> GSHMLEMIIKPRVRGFICVTAHPTGCEANVKKQIDYVTTEGPIANGPKRVLVIGASTGYGLAARITAAFGCGADTLGVFFERPGEEGKPGTSGWYNSAAFHKFAAQKGLYAKSINGDAFSDEIKQLTIDAIKQDLGQVDQVIYSLASPRRTHPKTGEVFNSALKPIGNAVNLRGLDTDKEVIKESVLQPATQSEIDSTVAVMGGEDWQMWIDALLDAGVLAEGAQTTAFTYLGEKITHDIYWNGSIGAAKKDLDQKVLAIRESLAAHGGGDARVSVLKAVVSQASSAIPMMPLYLSLLFKVMKEKGTHEGCIEQVYSLYKDSLCGDSPHMDQEGRLRA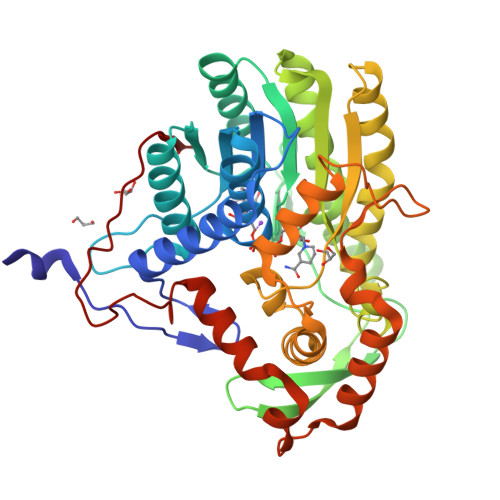DYKELDPEVQNQVQQLWDQVTNDNIYQLTDFVGYKSEFLNLFGFGIDGVDYDADVNPDVKIPNLIQG> MTLEKFVDALPIPDTLKPVQQSKEKTYYEVTMEECTHQLHRDLPPTRLWGYNGLFPGPTIEVKRNENV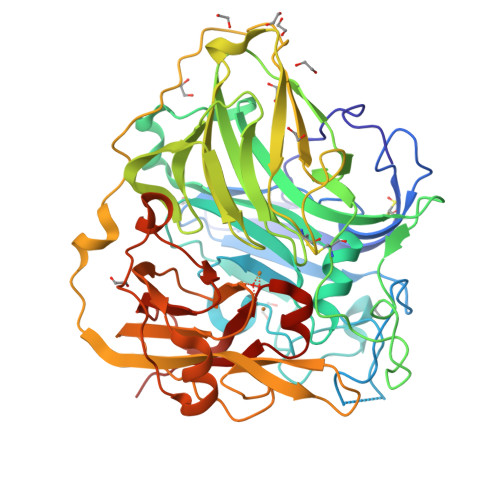YVKWMNNLPSTHFLPIDHTIHHSDSQHEEPEVKTVVHLHGGVTPDDSDGYPEAWFSKDFEQTGPYFKREVYHYPNQQRGAILWYHDHAMALTRLNVYAGLVGAYIIHDPKEKRLKLPSDEYDVPLLITDRTINEDGSLFYPSAPENPSPSLPNPSIVPAFCGETILVNGKVWPYLEVEPRKYRFRVINASNTRTYNLSLDNGGDFIQIGSDGGLLPRSVKLNSFSLAPAERYDIIIDFTAYEGESIILANSAGCGGDVNPETDANIMQFRVTKPLAQKDESRKPKYLASYPSVQHERIQNIRTLKLAGTQDEYGRPVLLLNNKRWHDPVTETPKVGTTEIWSIINPTRGTHPIHLHLVSFRVLDRRPFDIARYQESGELSYTGPAVPPPPSEKGWKDTIQAHAGEVLRIAATFGPYSGRYVWHCHILEHTDYDMMRPMDITDPHK>MKMVVVIRNDLGMGKGKMVAQGGHAIIEAFLDAKRKNPRAVDEWLREGQKKVVVKVNSEKELIDIYNKARSEGLPCSIIRDAGHTQLEPGTLTAVAIGPEKDEKIDKITGHLKLL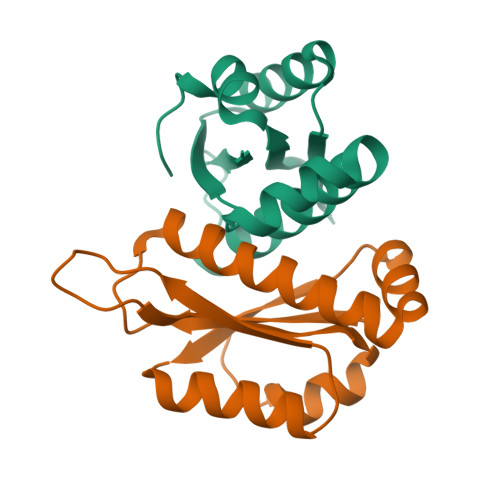[9x]Human ORP3 belongs to the oxysterol-binding protein (OSBP) family of lipid transfer proteins and is involved in lipid trafficking and cell signaling. ORP3 localizes to the ER-PM interfaces and is implicated in lipid transport and focal adhesion dynamics. The ORP3 ORD displays a helix grip β-barrel fold with a deep hydrophobic pocket which is conserved in the OSBP gene family. The ORP3 ORD has a central ligand-binding tunnel with a flexible lid covering the tunnel entrance.

The structures of the ORP3 ORDs in apo-form or in PI(4)P complex have a closed conformation of the lid by the hydrophobic interactions between the lid and the entrance of the hydrophobic tunnel. Structural comparison shows that the closed form of apo ORD has a very similar conformation to the PI(4)P-bound form with a Cα rmsd of 0.49 Å. The ligand dependent conformational change is limited to the residues that recognize the PI(4)P head group around the tunnel entrance. Two conserved arginine residues (residues 512–513) make salt bridges with the acidic loop β3-β4 and Glu794 in the groove formed by the β17-α6 and α6-α7 loops. Leu516 is accommodated in the hydrophobic pocket formed by helix α6 and the loop β17-α6. These interactions seem to stabilize the N-terminal base of the lid favoring a closed conformation of the lid. In contrast, the lid of Osh4 lacking the upstream residues is completely open and disordered when ligand is absent. In the asymmetric unit of the crystals, there were two molecules of ORP3 ORD related by two-fold non-crystallographic symmetry. The dimer in the asymmetric unit seemed to form by lattice interaction during crystallization process.

>[2x]GSPEFSGREAKSRRRTSLPAPSPSSSNISLWNILRNNIGKDLSKVAMPVELNEPLNTLQRLCEELEYSELLDKAAQIPSPLERMVYVAAFAISAYASSYYRAGSKPFNPVLGETYECIREDKGFQFFSEQVSHHPPISACHAESRNFVFWQDVRWKNKFWGKSMEIVPIGTTHVTLPVFGDHFEWNKVTSCIHNILSGQRWIEHYGEIVIKNLHDDSCYCKVNFIKAKYWSTNAHEIEGTVFDRSGKAVHRLFGKWHESIYCGGGSSSACVWRANPMPKGYEQYYSFTQFALELNEMDPSSKSLLPPTDTRFRPDQRFLEEGNLEEAEIQKQRIEQLQRERRRVLEENHVEHQPRFFRKSDGSWVSNGTYLELRKDLGFSKLDHPVLW> MPMVLLECDKDIPERQKHIYLKAPNEDTREFLPIANAATIPGTLSERGCAFCGAKLVIGGV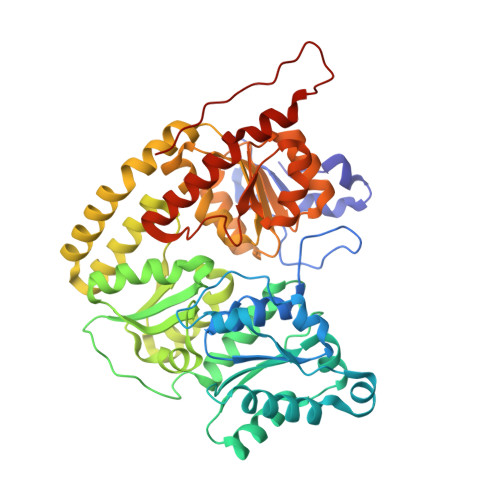LKDTIQMIHGPLGCAYDTWHTKRYPTDNGHFNMKYVWSTDMKESHVVFGGEKRLEKSMHEAFDEMPDIKRMIVYTTCPTALIGDDIKAVAKKVMKDRPDVDVFTVECPGFSGVSQSKGHHVLNIGWINEKVETMEKEITSEYTMNFIGDFNIQGDTQLLQTYWDRLGIQVVAHFTGNGTYDDLRCMHQAQLNVVNCARSSGYIANELKKRYGIPRLDIDSWGFNYMAEGIRKICAFFGIEEKGEELIAEEYAKWKPKLDWYKERLQGKKMAIWTGGPRLWHWTKSVEDDLGVQVVAMSSKFGHEEDFEKVIARGKEGTYYIDDGNELEFFEIIDLVKPDVIFTGPRVGELVKKLHIPYVNGHGYHNGPYMGFEGFVNLARDMYNAVHNPLRHLAAVDIRDKSQTTPVIVRGAA> RSSHHHHHHGEFDDPIRPPLKVARSPRPGQCQDVVQDVPNVDVQMLELYDRMSFKDIDGGVWKQGWNIKYDPLKYNAHHKLKVFVV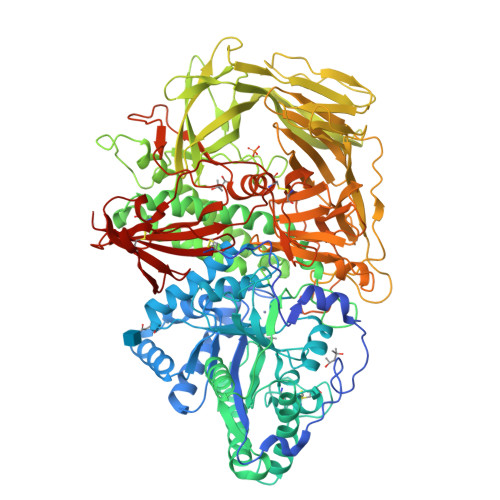PHSHNDPGWIQTFEEYYQHDTKHILSNALRHLHDNPEMKFIWAEISYFARFYHDLGENKKLQMKSIVKNGQLEFVTGGWVMPDEANSHWRNVLLQLTEGQTWLKQFMNVTPTASWAIAPFGHSPTMPYILQKSGFKNMLIQRTHYSVKKELAQQRQLEFLWRQIWDNKGDTALFTHMMPFYSYDIPHTCGPDPKVCCQFDFKRMGSFGLSCPWKVPPRTISDQNVAARSDLLVDQWKKKAELYRTNVLLIPLGDDFRFKQNTEWDVQRVNYERLFEHINSQAHFNVQAQFGTLQEYFDAVHQAERAGQAEFPTLSGDFFTYADRSDNYWSGYYTSRPYHKRMDRVLMHYVRAAEMLSAWHSWDGMARIEERLEQARRELSLFQHHDGITGTAKTHVVVDYEQRMQEALKACQMVMQQSVYRLLTKPSIYSPDFSFSYFTLDDSRWPGSGVEDSRTTIILGEDILPSKHVVMHNTLPHWREQLVDFYVSSPFVSVTDLANNPVEAQVSPVWSWHHDTLTKTIHPQGSTTKYRIIFKARVPPMGLATYVLTISDSKPEHTSYASNLLLRKNPTSLPLGQYPEDVKFGDPREISLRVGNGPTLAFSEQGLLKSIQLTQDSPHVPVHFKFLKYGVRSHGDRSGAYLFLPNGPASPVELGQPVVLVTKGKLESSVSVGLPSVVHQTIMRGGAPEIRNLVDIGSLDNTEIVMRLETHIDSGDIFYTDLNGLQFIKRRRLDKLPLQANYYPIPSGMFIEDANTRLTLLTGQPLGGSSLASGELEIMQDRRLASDDERGLGQGVLDNKPVLHIYRLVLEKVNNCVRPSKLHPAGYLTSAAHKASQSLLDPLDKFIFAENEWIGAQGQFGGDHPSAREDLDVSVMRRLTKSSAKTQRVGYVLHRTNLMQCGTPEEHTQKLDVCHLLPNVARCERTTLTFLQNLEHLDGMVAPEVCPMETAAYVSSHSS>[10x]DEIKIVKYPDPILRRRSEEVTNFDDNLKRVVRKMFDIMYESKGIGLSAPQVNISKRIIVWNALYEKRKEENERIFINPSIVEQSLVKLKLIEGCLSFPGI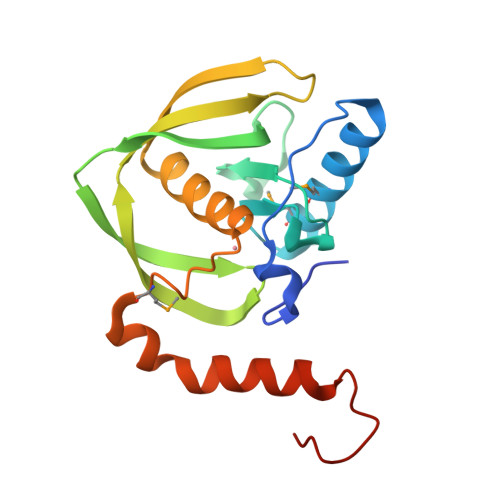EGKVERPSIVSISYYDINGYKHLKILKGIHSRIFQHEFDHLNGTLFIDKMTQVDKKKVRPKLNELIRDYKATHSEEPLEHHHHHH>[2x]MEMMIKKRIKQVKKGDQDAFADIVDIYKDKIYQLCYRMLGNVHEAEDIAQEAFIRAYVNIDSFDINRKFSTWLYRIATNLTIDRIRKKKPDYYLDAEVAGTEGLTMYSQIVADGVLPEDAVVSLELSNTIQQKILKLPDKYRTVIVLKYIDELSLIEIGEILNIPVGTVKTRIHRGREALRKQLRDL;>[2x]MSCPEQIVQLMHMHL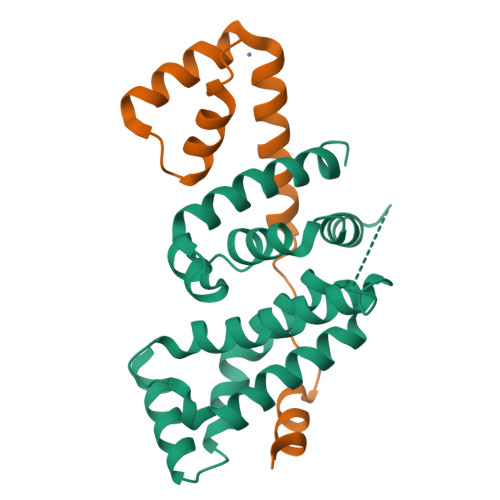DGDILPKDEHVLNEHLETCEKCRKHFYEMEKSIALVRSTSHVEAPADFTANVMAKLPKEKKRASV> MAPVTNGRIIFNSIPTGFPVPGETTIYDTTETIDLDTAPLDGGFLLKTLELSVDPYMRGGMRAPEKKSYSAPFTLGQPLRGYGVGVVLRSENPQVKAGDHLYGFFEHTHYSIRKDLTGLQAIENAYNLPWSVFIGVIGMPGKTAYMAWKEYAHPKQGETVFVSTGAGPVGSFVIQLAKADGLKVIASAGSEEKVQFMKEVGADVAFNYKTTNTAEVLEKEGPIDIYWDNVGGETLEAALNAANVNARFIECGMISGYNSGGAPVRNIFHVIGKSITMTGFIVSRIEPKYSAEFYKEVPAKVASGELKYREHVYNGLEKLGDVILAVQKGENKAKAVVHVADDLEHHHHH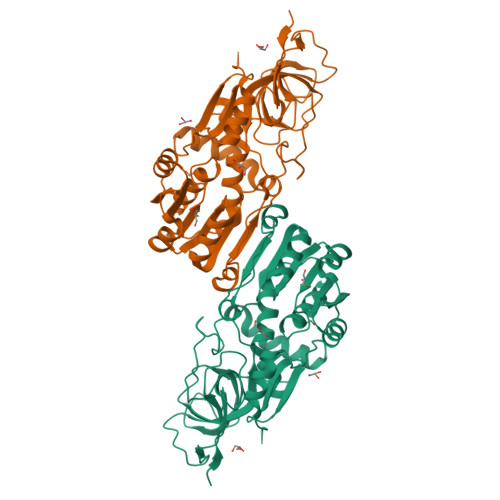H> LNRLREPLLRRLSELLDQAPEGRGWRRLAELAGSRGRLRLSCLDLEQCSLKVLEPEGSPSLCLLKLMGEKGCTVTELSDFLQAMEHTEVLQ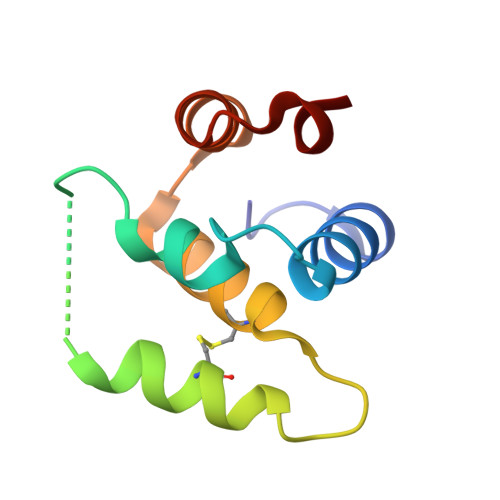L[(2~{S},7~{S},11~{S},15~{S},19~{R},22~{R},26~{S},30~{R},34~{R},38~{S},43~{S},47~{S},51~{S},55~{R},58~{R},62~{S},66~{R},70~{R})-38-(hydroxymethyl)-7,11,15,19,22,26,30,34,43,47,51,55,58,62,66,70-hexadecamethyl-1,4,37,40-tetraoxacyclodoheptacont-2-yl]methanol 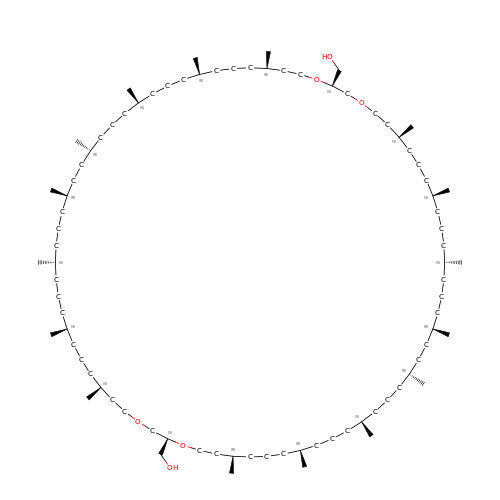| C86 H172 O6 | VMHUDYKDOMRJOK-PFTGJOHNSA-N> KEIPEVLVDPRSRRRYVRGRFLGKGGFAKCFEISDADTKEVFAGKIVPKSLLLKPHQREKMSMEISIHRSLAHQHVVGFHGFFE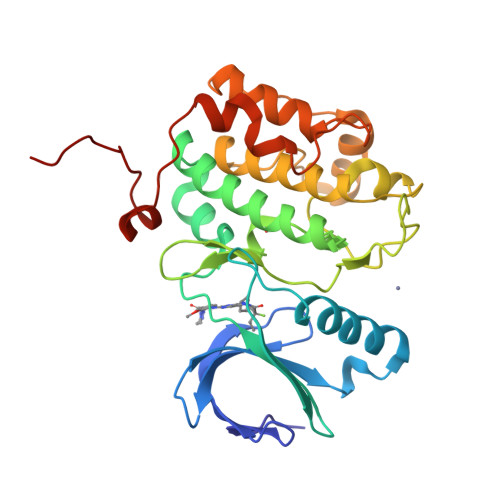DNDFVFVVLELCRRRSLLELHKRRKALTEPEARYYLRQIVLGCQYLHRNRVIHRDLKLGNLFLNEDLEVKIGDFGLATKVEYDGERKKVLCGTPNYIAPEVLSKKGHSFEVDVWSIGCIMYTLLVGKPPFETSCLKETYLRIKKNEYSIPKHINPVAASLIQKMLQTDPTARPTINELLNDEFFTSGYIPARLPITCLTIPPRFSIAPS> MANQRMLGFVHTAQRMPDKRPAAERRQDFAEIYARFSDERANEQANRCSQCGVPFCQVHCPVSNNIPDWLKLTSEGRLEEAYEVSQATNNFPEICGRICPQDRLCEGNCVIEQSTHGAVTIGSVEKYINDTAWDQGWVKPRTPSRELGLSVGVIGAGPAGLAAAEELRAKGYEVHVYDRYDRMGGLLVYGIPGFKLEKSVVERRVKLLADAGVIYHPNFEVGRDASLPELRRKHVAVLVATGVYKARDIKAPGSGLGNIVAALDYLTTSNKVSLGDTVEAYENGSLNAAGKHVVVLGGGDTAMDCVRTAIRQGATSVKCLYRRDRKNMPGSQREVAHAEEEGVEFIWQAAPEGFTGDTVVTGVRAVRIHLGVADATGRQTPQVIEGSEFTVQADLVIKALGFEPEDLPNAFDEPELKVTRWGTLLVDHRTKMTNMDGVFAAGDIVRGA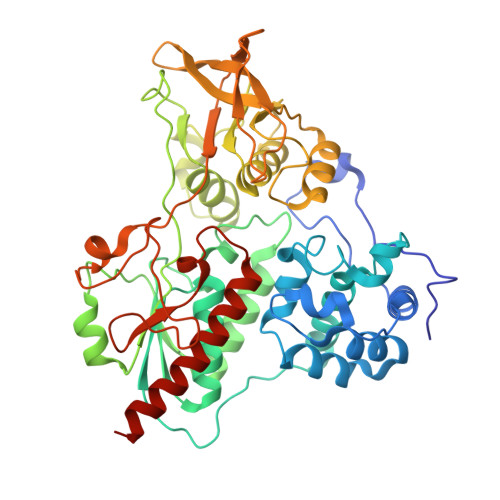SLVVWAIRDGRDAAEGIHAYAKAKAEAPVAVAAE> MSLRRGIYHIENAGVPSAIDLKDGSSSDGTPIVGWQFTPDTINWHQLWLAEPIPNVADTFTLCNLFSGTYMDLYNGSSEAGTAVNGWQGTAFTTNPHQLWTIKKSSDGTSYKIQ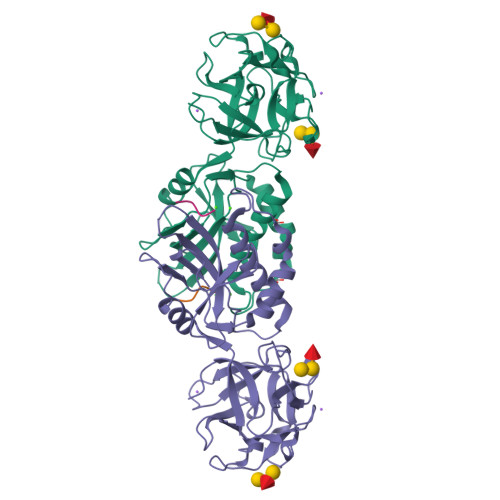NYGSKTFVDLVNGDSSDGAKIAGWTGTWDEGNPHQKWYFNRMSVSSAEAQAAIARNPHIHGTYRGYILDGEYLVLPNATFTQIWKDSGLPGSKWREQIYDADDFAIAMKAAVGKWGADSWKANGFAIFCGVMLGVNKAGDAAAAYNFTLTKDHADIVFFEPQNGGYLNDIGYDSYMAFY;> PVVR> AAYFQGAASTVKVTEQLRH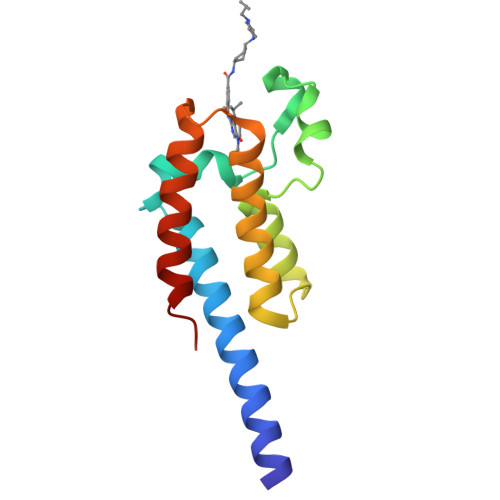CSEILKEMLAKKHFSYAWPFYNPVDVNALGLHNYYDVVKNPMDLGTIKEKMDNQEYKDAYKFAADVRLMFMNCYKYNPPDHEVVTMARMLQDVFETHFSKIPI methyl 4-sulfanylbenzoate | C8 H8 O2 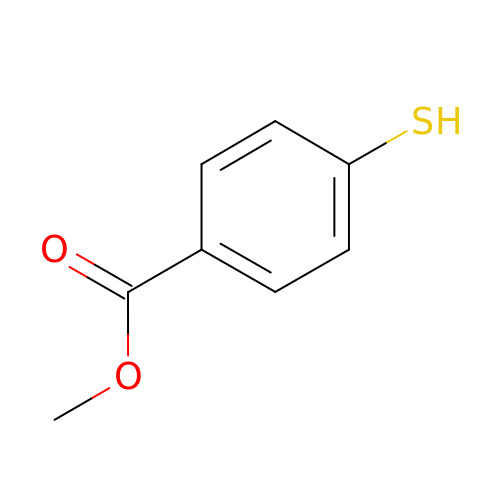S | BTZOMWXSWVOOHG-UHFFFAOYSA-N> XELEAIAQKFEAIAKKFEAIAFKFEAIAQKX;> XELKAI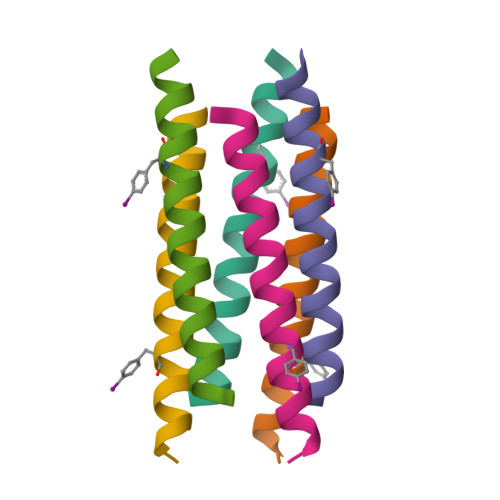AQEFKAIAKEFKAIAFEFKAIAQKX In plant cells, ALMTs are key plasma and vacuolar membrane-localized anion channels regulating plant responses to the environment. Among the different ion transporters and ion channels localized in the vacuolar membrane, the ion channels of the aluminum-activated malate transporter (ALMT) family play a key role for the transport of chloride and malate during stomata opening/closure. ALMTs are also involved in transporting various anion including chloride, nitrate, fumarate, tartrate, citrate, and malate. Here we report the cryo-EM structures of ALMT9 from Arabidopsis thaliana (AtALMT9), a malate-activated vacuolar anion channel, in plugged and unplugged lipid-bound states.

From the CHS-supplemented dataset 1 with no malate and dataset 2 with 10 mM malate, we unequivocally identified CHS densities in the lateral fenestrations and phospholipid (PL) densities in the pore (hereinafter called as “pore lipid”) in two classes. The only difference observed between the datasets 1 and 2 was the presence of a malate density in the pore of the dataset 2. In the CHS-supplemented datasets 1 and 2, we identified two distinct classes in the sterol mimic-bound state: “sterol 1” when one pore lipid tail of the sterol mimic (CHS) is in the fenestrations and “sterol 2” when two pore lipid tails of the sterol mimic (CHS) are in the fenestrations. Unexpectedly, we observed that the succinate head group of CHS interacted with several residues. Since the succinate group was the key structural moiety to differentiate CHS from native cholesterols, these interactions were likely to present artificial features and to inhibit pore lipid expulsion (described later). Similarly, the succinate head group of CHS in the lower fenestrations occupied the S3 region interacting with W120, Y208, and R226. These observations indicate that phosphate groups of PL and the dicarboxylic moieties (malate and succinate head group of CHS) compete with each other for malate binding sites S0, S1, and S3. The sterol mimic-bound and pore lipid-bound classes represent plugged states in which the pore is blocked by the head groups of one or two pore lipids. Additionally, the TMD of the sterol mimic-bound classes is similar with those of the pore lipid-bound and peripheral lipid-bound classes, suggesting that plant sterols may contribute to the regulation of the clade 2 ALMTs.

>[2x]MAAKQGSFRHGILEKRERLLSNNGFSDFRFTDIESNDLLENENCGRRTRLCCCCSCGNLSEKISGVYDDAKDVARKAWEMGVSDPRKIVFSAKIGLALTIVALLIFYQEPNPDLSRYSVWAILTVVVVFEFTIGATLSKGFNRALGTLSAGGLALGMAELSTLFGDWEEIFCTLSIFCIGFLATFMKLYPSMKAYEYGFRVFLLTYCYILISGFRTGQFIEVAISRFLLIALGAGVSLGVNMFIYPIWAGEDLHNLVVKNFMNVATSLEGCVNGYLRCLEYERIPSKILTYQASEDPVYKGYRSAVESTSQEESLMSFAIWEPPHGPYKSFNYPWKNYVKLSGALKHCAFTVMALHGCILSEIQAPEERRQVFRQELQRVGVEGAKLLRELGEKVKKMEKLGPVDLLFEVHLAAEELQHKIDKKSYLLVNSECWEIGNRATKESEPQELLSLEDSDPPENHAPPIYAFKSLSEAVLEIPPSWGEKNHREALNHRPTFSKQVSWPARLVLPPHLETTNGASPLVETTKTYESASALSLATFASLLIEFVARLQNVVDAFKELSQKANFKEPEIVTTGTDVEFSGERVGLGQKIRRCFGM> ASNL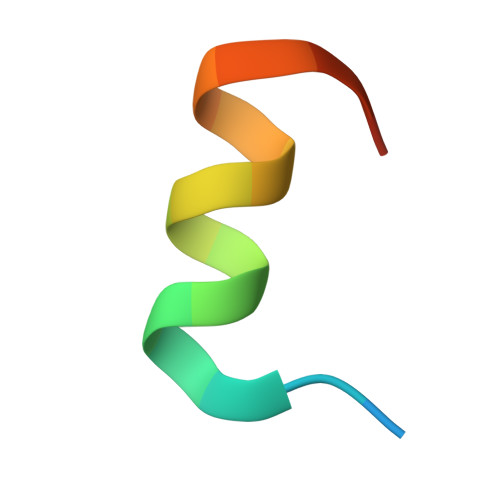GLEDIIRKALMGSFD> MAHAGRTGYDNREIVMKYIHYKLSQRGYEWDAGDDVEENRTEAPEGTESEVVHLTLRQAGDDFSRRYRRDFAEMSSQLHLTPFTARGRFATVVEELFRDGVNWGRIVAFFEFGGVMCVESVNREMSPLVDNIALWMTEYLNRHLHTWIQDNGGWDAFVELYGPS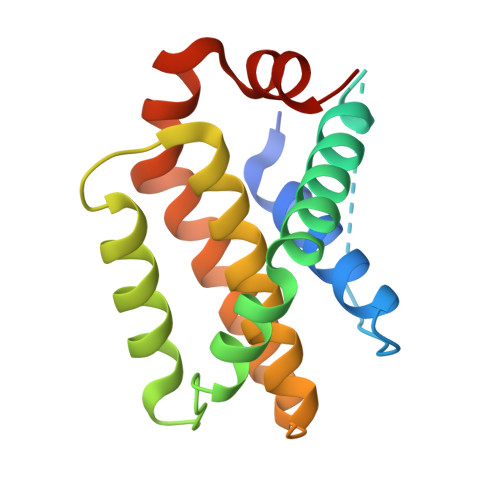MR>MNIVVLISGNGSNLQAIIDACKTNKIKGTVRAVFSNKADAFGLERARQAGIATHTLIASAFDSREAYDRELIHEIDMYAPDVVVLAGFMRILSPAFVSHYAGRLLNIHPSLLPKYPGLHTHRQALENGDEEHGTSVHFVTDELDGGPVILQAKVPVFAGDSEDDITARVQTQEHAIYPLVISWFADGRL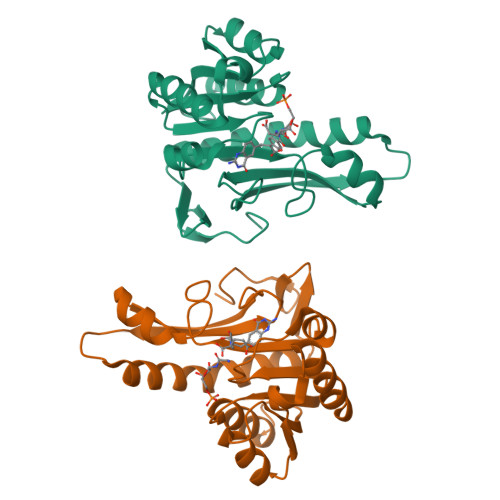KMHENAAWLDGQRLPPQGYAADE[2x]> MATDLKASSLRALKLMHLATANDDDTDENVIALCHQAKTPVGNTDAIFIYPRFIPIARKTLKEQGTPEIRICTSTNFPHGNDDIDIALAETRAAIAYGADSVAVVFPYRALMAGNEQVGFDLVKACKEACAAANVLLAVIIETGELKDEALIRK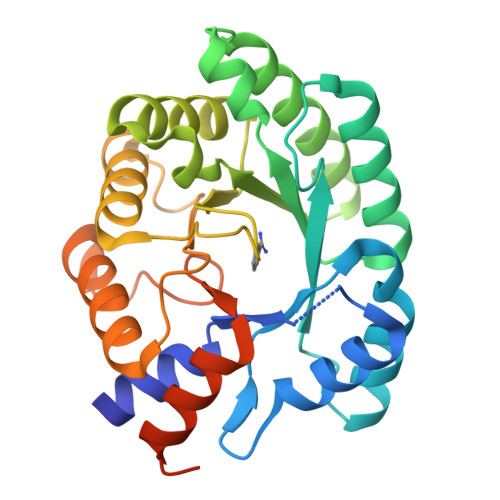ASEISIKAGADNIVTSTPGKVAEGATPESARIMMEVIRDMGVEKTVGFIPVGGVRTAEDAQKYLAIADELFGADWADSRHYAFGASSSLLASLLKALGHGDGKSASSYGSLEHHHHHH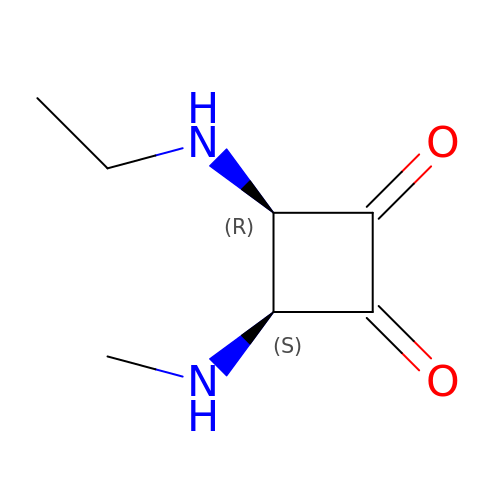3-ETHYLAMINO-4-METHYLAMINO-CYCLOBUTANE-1,2-DIONE | C7 H12 N2 O2 | FYAIPBIOBLLUAM-UHFFFAOYSA-N>GAMGSNGRQLLEELRKDEELRRALAEELIPEVLRNRELRRAILLALSREMATKEDIEALRKATKEDIEDLREATKEDIEALRKATKEDIEALREDIEALRKATK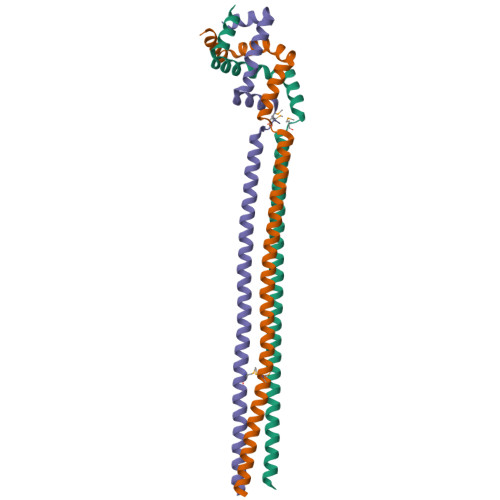ENMEKLEAELKSYVDARVIELKSYIDTRLDSINER[3x]> MENTENSVDSKSIKNLEPKIIHGSESMDSGISLDNSYKMDYPEMGLCIIINNKNFHKSTGMTSRSGTDVDAANLRETFRNLKYEVRNKNDLTREEIVELMRDVS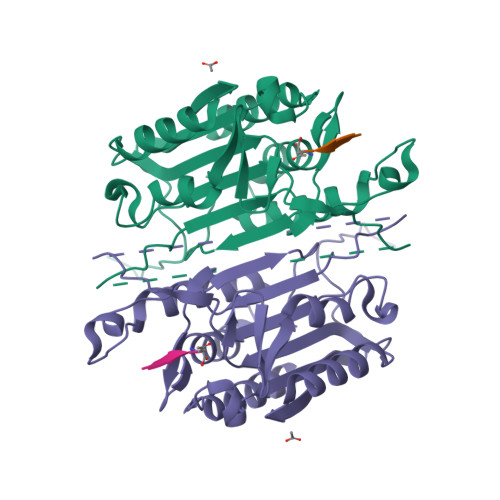KEDHSKRSSFVCVLLSHGEEGIIFGTNGPVDLKKITNFFRGDRCRSLTGKPKLFIIQACRGTELDCGIETDSGVDDDMACHKIPVEADFLYAYSTAPGYYSWRNSKDGSWFIQSLCAMLKQYADKLEFMHILTRVNRKVATEFESFSFDATFHAKKQIPCIHSMLTKELYFYH>[4x]MNEFTAVKELSEKLLEDYKTESSLFFASPTRTILAEGEFTTVKHHEIESFPELVQAVLRNAKQAGNPNPIVVGALPFDRRKEVQLIVPEYSRISERLQLDPTNHLEINRNLTFEMTPVPDHEVYMKGVKQGIEKIKDGDLKKIVLSRSLDVKSSGKID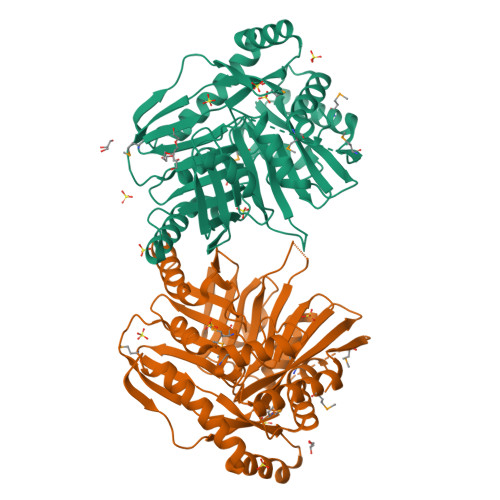KQKLLRELAEHNKHGYTFAVNLPKDENENSKTLIGASPELLVSRHGMQVISNPLAGSRPRSDDPVEDKRRAEELLSSPKDLHEHAVVVEAVAAALRPYCHTLYVPEKPSVIHSEAMWHLSTEVKGELKNPNTSSLELAIALHPTPAVCGTPMEEAREAIQKIEPFDREFFTGMLGWSDLNGDGEWIVTIRCAEVQENTLRLYAGAGVVAESKPEDELAETSAKFQTMLKALGLNDSSLNEK Mupirocin, a clinically used natural antibiotic, inhibits isoleucyl-tRNA synthetase (IleRS), an enzyme that links isoleucine to its tRNAIle for protein synthesis. Two IleRSs, mupirocin-sensitive IleRS1 and resistant IleRS2, coexist in bacteria. Specifically, type 1 proteins (IleRS1) are strongly inhibited by mupirocin (Ki in low nanomolar range), while IleRS2, which are homologous to IleRSs from the eukaryote cytosol, exhibit resistance to mupirocin concentrations that are about three orders of magnitude higher. AARSs catalyze the formation of AA-tRNA in two steps within the same active site. The amino acid is first activated by ATP to form an aminoacyl-adenylate (AA-AMP) intermediate, followed by the transfer of the aminoacyl moiety to the tRNA.

Therefore, to deepen our understanding of mupirocin resistance in general and to infer the mechanism of hyper-resistance, we determined the crystal structures of wild-type PmIleRS1 (sensitive) and PmIleRS2 (resistant), both of which carry the canonical HXGH motif and are amenable in mupirocin-bound form when the inhibitor is supplied at sufficiently high concentrations. To alleviate this problem, we solved the structures of IleRS1 (sensitive) and IleRS2 (resistant) from P. megaterium bound to mupirocin only. The structures provide an important progress in understanding the resistance mechanism by identifying that the closed conformation of the active site KMSKS loop in IleRS2 precludes H-bonding stabilization of the mupirocin’s carboxylate. In PmIleRS2, the closed conformation of the KMSKS loop forces binding of the nonanoic carboxylate such that it is positioned at 4.1 Å distance to the NH of Lys593 (KMSKS). It is this lack of carboxylate stabilization by H-bonding that may strongly affect the IleRS2 affinity towards mupirocin and provide resistance. Interestingly, we observed a kink of helix α2 (from residues 123–126) solely in the crystal structure of mupirocin-bound PmIleRS2. Thus, the MD data suggest that the kink in helix α2 is part of the conformational flexibility of IleRS2 and is neither induced by mupirocin binding nor by different packing environments in the different space groups that PmIleRS2:mupirocin and PmIleRS2:Ile-AMS crystallized in. Structural data unraveled that in the PmIleRS2:mupirocin complex, the tip of the helix α1 carrying the HXGH motif is shifted back towards helix α2, resulting in 2.9 or 3.3 Å displacements of the first or fourth His, respectively, relative to PmIleRS2:Ile-AMS. Thus, in the PmIleRS2:mupirocin complex the HXGH motif adopts the same position as in the IleRS1 structures. The back-shift of the HIGH motif is likely promoted by binding of the nonanoic part of mupirocin to the channel between the HIGH motif and the KMSKS loop forced by the closed conformation of the KMSKS loop in PmIleRS2.

> MKEVNVRESSQEREQRIQQQWQKGNVFQQSVQNREGYPSFVFYEGPPTANGLPHVGHALGRTIKDVVARYKTMTGHQVIRKAGWDTHGLPVELGVEKQLGISGKHDIEKYGVEAFINKCKESVFVYEKQWRTFTEQLGYWVDMEDPYITLENSYIESVWNVLGTIHDKGLLYKGHRVSPYCPSCQTSLSSHEVAQGYKDVKDLTVTVKFKVKNRDNEYFLGWTTTPWTLPSNVALAVHEEMSYVRAEQGDSVYIVAEALADKVLKGEYSVLSHHKGNELKGMSYEPPFNFVKVEKGHEVVTADYVTDQSGTGVVHLAPAYGEDDYRVVKENGFSFVNVVDEKGQYTSEVPPFQGRFVKDCDVDIVRYLANQDVLYHKEKHEHSYPFCWRCDSPLLYYANESWFIQTTALKEQFLKNNESVKWYPDHIKHGRFGKFLENMVDWNISRKRYWGTPLNVWECEGCQHQVAPKSIKELQKHASHYVDDSIELHKPYVDDVQLTCPVCSGEMKRTPEVIDVWFDSGSMPFAQYHYPFENSELFQKQFPADVIAEGIDQTRGWFYSLMAVSTLFTGKAPYKRVLSLGHVLDENGQKMSKSKGNALDPVDLIHTFGADALRWALLADSAPWNPKKFSERVVQEAKSKVIDTLVNVYGFYVLYAKLDGYDPEQTYELKKTKLDEWILSRLHSTVKRATVHLEDYGFTSAAREIAVFIEELSNWYVRRSRDRFWSEGMDGEKAAAYDTLHEVLVTLSQLLAPFTPFVADDVHENLTGKSVHLADYPACDQTKVNEKLEKEMAAVLQVVELGRSIRNTHSLKVKQPLQSLSLVVTEEDVEWKAYRDVIKDELNVKNFNVEQDDDKVLSYVLKLDFKQAGPKFGKQVNEVNQALKNLSEEKGKEFVEQGKLSVTLASGENLTLETEDVLVEKVPKEGFAVASNGMYTAVLDTALTEELVQEGVAREVIRAVQDYRKKLDLPVNSRINLELSGDEEVQKAVAKFETLLQENLLLHSLSVKETIKNGETVKVGTKQVVLRVLNQS> YQQDQVVKEDNIEAVGKKLHEYN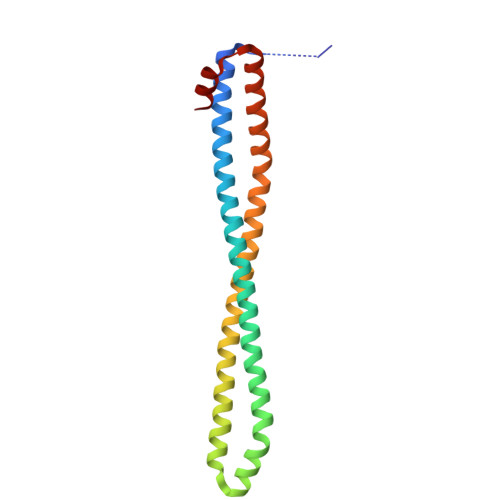TQFQEKSREYDRLYEDYTRTSQEIQMKRTAIEAFNETIKIFEEQCQTQERYSKEYIEKFKREGNETEIQRIMHNYEKLKSRISEIVDSRRRLEEDLKKQAAEYREIDKRMNSIKPDLIQLRKTRDQYLMWLTQKGVRQKKLNEWLGN> MHHHHHHMNPERSERIEIPVLPLRDVVVYPHMVIPLFVGREKSIRCLEAAMDHDKKIMLVAQKEASTDEPGVNDLFTVGTVASILQMLKLPDGTVKVLVEGLQRARISALSDNGEHFSAKAEYLESPTIDEREQEVLVRTAISQFEGYIKLNKKIPPEVLTSLNSIDDPARLADTIAAHMPLKLADKQSVLEMSDVNERLEYLMAMMESEIDLLQVEKRIRNR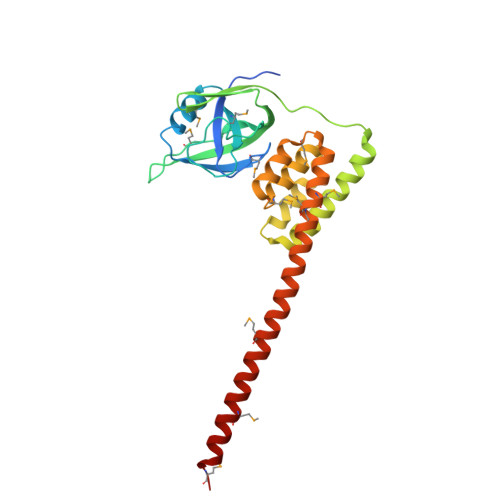VKKQMEKSQREYYLNEQMKAIQKELGEMD>[2x]MSKTQEFRPLTLPPKLSLSDFNEFIQDIIRIVGSENVEVISSKDQ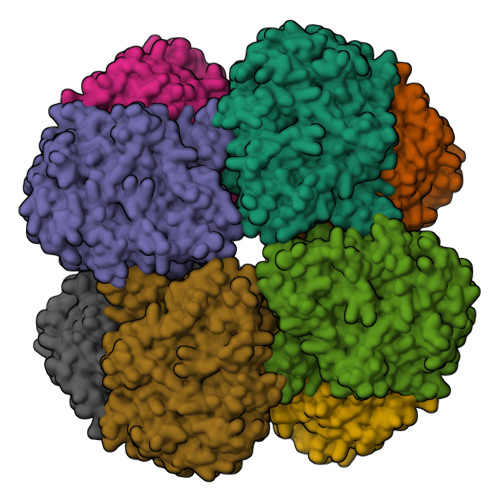IVDGSYMKPTHTHDPHHVMDQDYFLASAIVAPRNVADVQSIVGLANKFSFPLWPISIGRNSGYGGAAPRVSGSVVLDMGKNMNRVLEVNVEGAYCVVEPGVTYHDLHNYLEANNLRDKLWLDVPDLGGGSVLGNAVERGVGYTPYGDHWMMHSGMEVVLANGELLRTGMGALPDPKRPETMGLKPEDQPWSKIAHLFPYGFGPYIDGLFSQSNMGIVTKIGIWLMPNPRGYQSYLITLPKDGDLKQAVDIIRPLRLGMALQNVPTIRHILLDAAVLGDKRSYSSRTEPLSDEELDKIAKQLNLGRWNFYGALYGPEPIRRVLWETIKDAFSAIPGVKFYFPEDTPENSVLRVRDKTMQGIPTYDELKWIDWLPNGAHLFFSPIAKVSGEDAMMQYAVTKKRCQEAGLDFIGTFTVGMREMHHIVCIVFNKKDLIQKRKVQWLMRTLIDDCAANGWGEYRTHLAFMDQIMETYNWNNSSFLRFNEVLKNAVDPNGIIAPGKSGVWPSQYSHVTWKL>MAEVIRSSAFWRSFPIFEEFDSETLCELSGIASYRKWSAGTVIFQRGDQGDYMIVVVSGRIKLSLFTPQGRELMLRQHEAGALFGEMALLDGQPRSADATAVTAAEGYVIGKKDFLALITQRPKTAEAVIRFLCAQLRDTTDRLETIALYDLNARVARFFLATLRQIHGSEMPQSANLRLTLSQTDIASILGASRPKVNRAILSLEESGAIKRADGIICCNVGRLLSIADPEEDLEHHHHHHHH[2x]

In contrast, both cyclic nucleotides mediate transcription activation by Sinorhizobium meliloti Clr, mapping to cluster G of Crp-like proteins. We present crystal structures of Clr-cAMP and Clr-cGMP bound to the core motif of the palindromic Clr DNA binding site (CBS). The structures show a Clr dimer that is bound to CBS-DNA. The individual subunits fold into two domains linked by helix α5 (residues P123 to L149), which is the Clr dimerization interface.

The cNMP binding site located in the N-terminal domain is stoichiometrically occupied by cAMP and cGMP, respectively. The binding modes of the phosphate and sugar moieties are identical, involving G85 and E86 within α4 as well as R95 and S96 of the following loop. The nucleobase of cGMP is flipped to the syn conformation, while it occupies the anti conformation in the Clr-cAMP complex. While cAMP interacts via its primary N6-amine with both T140 and T141, cGMP forms hydrogen bonds between T140 and its C-6 carbonyl group as well as between T141 and the N2-amine. Interaction of the cAMP nucleotide with both α5 helices has been described to trigger a coil-to-helix transition in the C-terminal part of the hinge and to shift the HTH domain toward its active conformation for CAP. In the case of Clr, both the interaction and arrangement of the full α5 helix are resolved by the structure, which is in an agreement with Clr-DNA binding in vitro and activation of promoter activity in vivo by both cNMPs. The affinity of cAMP binding itself by Clr is mostly not affected by the presence of cognate CBS-DNA with equilibrium dissociation constant (KD) values of 6 to 7 μM. Formation of the ternary Clr–cAMP–CBS-DNA complex is enthalpically driven with an opposed loss of entropy, whereas that of the binary Clr-cAMP complex relies both on enthalpic and entropic contributions. The relative hydrogen-deuterium exchange comparing the apo and holo states also shows a slightly stronger decline in deuterium uptake within the binding pocket for the cAMP-bound state than for the cGMP-bound state. Furthermore, Clr-cAMP produced stronger band shifts than Clr-cGMP.>MVDMSKVKLRIENIVASVDLFAQLDLEKVLDLCPNSKYNPEEFPGIICHLDDPKVALLIFSSGKLVVTGAKSVQDIERAVAKLAQKLKSIGVKFKRAPQIDVQNMVFSGDIGREFNLDVVALTLPNCEYEPEQFP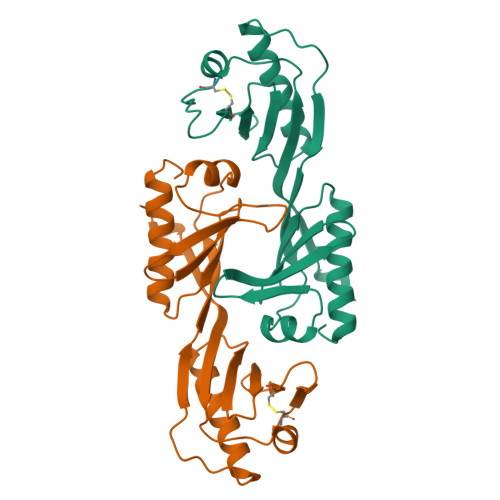GVIYRVKEPKSVILLFSSGKIVCSGAKSEADAWEAVRKLLRELDKYGLLEEEEEEL[2x]> MLRRRVLPESHRHASWPLIYETSQHGIKTLDVREYRPLATPIEFRFYQRYANHPNRQSGIQFLTHYNTHQRFRVNKDYIDYMHWGKEQGQARLPHRHQRVAFDFDDQLHPTRTLDNEGDSYAWCAEQDPTLGPHPDLDASFDPNRRVFSHPEHWNKMFSKRRPGEGRIDLRVLPSQSLLGPLMEQSDTQGAAYFRYDNRGHSNGRVPGLNTPFFGEFDRKMMQAMSRPLNADRTITGNDGRFSKTIMINEPKTHQALSGKTASELSVEIDKATNAVHSKLTVLEAAQSGLTNYYCGGLNFEMLGFDLHMAEMLREKARAILNGVASVSSTSVMVTTTSVPTKAQEREVGQLLRDALRYEDRVDDAIRQHASLIWRVYTAPRPLMALTNGKCRGTGCGVSLYSKYCALKDASEFIFDGPNLGITPYGGLTRLLARPETSLKYPGLAEFIMLTGTSLFAGDALRLGWTDLFTTLPDMSYHIKDWFDTTEHMHNDAVAWQLGHLLETCFKMKEAHSSAMERVAITPVRARWIEDSFADQPSVNHIINTLSEIERLPITAKQNTCDQTRCTPYTLTSVEAGISKLENHRLRYTHSPWDITPPEDEVSLQHASEIFNAYVLERRGTFNVVVHRDTEKLAAWNRQRQEEYHAYRSLRAAPHPRHVYARLEGCEGKLVSFDFVFSLQGKQKDQRSGNKEGEELQQTACLDALKRQVLTSFGMPDGRDIELGWYLPTLDTCPIHNDVEIMQLLHADPGIEDPKAQLKYPPIYFIVKRNCLYFSEWAYAVKHQLLLQSPFALRAAYEMLLEVRGDGSAERVMPLAESLATEFKYISRLLRRPDFYRVGVHTDKSAEAWEEIREERQRNLHKTHQPTRPLPDFEDVFERNVEIDGHRFLLRPRWSPRTLQEVLDADVMRLHTSLAYQDEGIAPLHVPTQCAKANRISDMVEDAGGLEVVPGLGELDAKGTPVVPPLQSNAHVPQNVSFYEMARHPWEDAASSWRRDGFTEGSLANYEAQYRAAERAVYDEEGRGGHNYWPSRE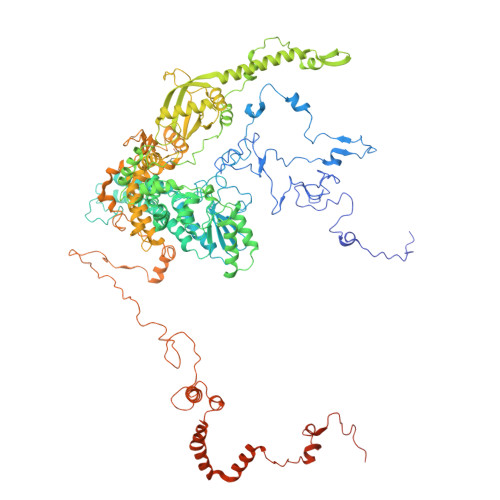ASEGVTSEEKDAALLRERLFKPLEEALSGVEPWARNLRRSASDGKLGYKTEIATPEEKIYDDEYYRWFIQPGHHPNPTGLTNVHKGSSTLQGSDAAEFERIWRHVVSGVDGGNASDEAETAAEDGEEEGDTQMNEKNPVVPNDEEEGV>[4x]MAAADGDDSLYPIAVLIDELRNEDVQLRLNSIKKLSTIALALGVERTRSELLPFLTD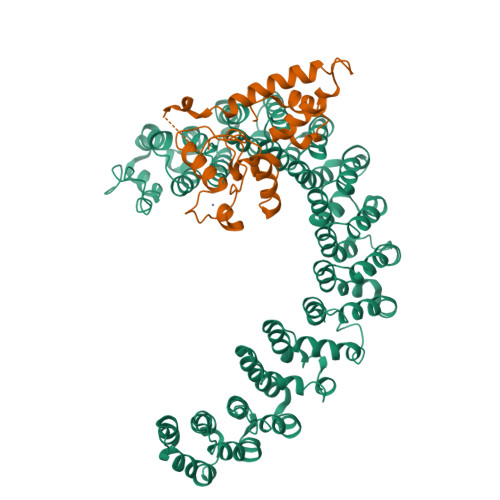TIYDEDEVLLALAEQLGTFTTLVGGPEYVHCLLPPLESLATVEETVVRDKAVESLRAISHEHSPSDLEAHFVPLVKRLAGGDWFTSRTSACGLFSVCYPRVSSAVKAELRQYFRNLCSDDTPMVRRAAASKLGEFAKVLELDNVKSEIIPMFSNLASDEQDSVRLLAVEACVNIAQLLPQEDLEALVMPTLRQAAEDKSWRVRYMVADKFTELQKAVGPEITKTDLVPAFQNLMKDCEAEVRAAASHKVKEFCENLSADCRENVIMTQILPCIKELVSDANQHVKSALASVIMGLSPILGKDNTIEHLLPLFLAQLKDECPEVRLNIISNLDCVNEVIGIRQLSQSLLPAIVELAEDAKWRVRLAIIEYMPLLAGQLGVEFFDEKLNSLCMAWLVDHVYAIREAATSNLKKLVEKFGKEWAHATIIPKVLAMSGDPNYLHRMTTLFCINVLSEVCGQDITTKHMLPTVLRMAGDPVANVRFNVAKSLQKIGPILDNSTLQSEVKPILEKLTQDQDVDVKYFAQEALTVLSLA;>MDKVLNREESLQLMDLLGLERSAWGNIPLMRKAYLKKCKEFHPDKGGDEEKMKKMNTLYKKMEDGVKYAHQPDFGGFWDATEVFASSLNPGVDAIYCKQWPECVKKMSTNCICLLCLLRMKHENRKLYRKDPLVWVDCYCFDCFRMWFGLDLCEGTLLLWCDIIGQTTYRDLKL[4x]> DTSGVQGIDVSHWQGSINWSSVKSAGMSFAYIKATEGTNYKDDRFSANYTNAYNAGIIRGAYHFARPNASSGTAQADYFASNGGGWSRDNRTLPGVLDIEHNPSGAMCYGLSTTQMRTWINDFHARYKARTTRDVVIYTTASWWNTCTGS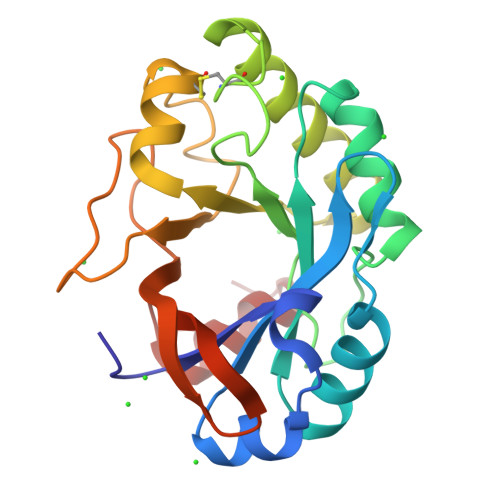WNGMAAKSPFWVAHWGVSAPTVPSGFPTWTFWQYSATGRVGGVSGDVDRNKFNGSAARLLALANNTA>[2x]GVKAKVLENFLTKSRTELLEYFVKVIFDYNTAHNKVSLSNKYTTASVSDGLQHYRSH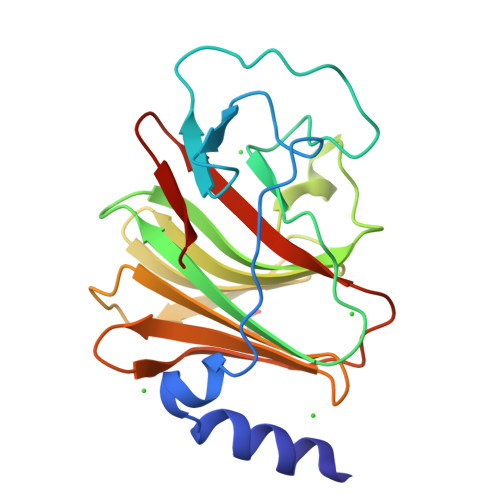PQRFTYCSQVLGLHCYKNGIHYWEVELQKNNFCGVGICYGSMERQGPESRLGRNPNSWCVEWFNNKISAWHNNVEKTLPSTKATRVGVLLNCDHGFVIFFAVTEKVHLMYKFKVDFTEALYPAFWVFSAGTTLSICSK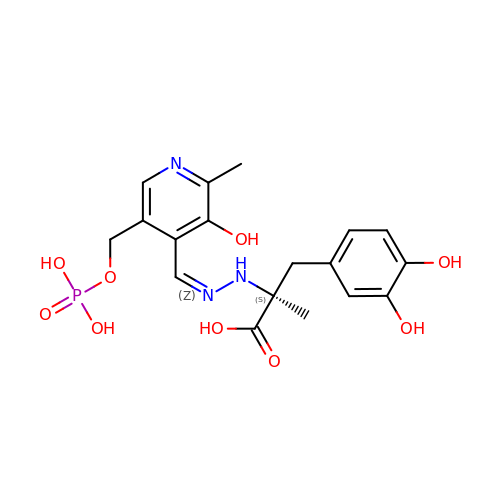(2S)-3-(3,4-dihydroxyphenyl)-2-[(2E)-2-({3-hydroxy-2-methyl-5-[(phosphonooxy)methyl]pyridin-4-yl}methylidene)hydrazin-1-yl]-2-methylpropanoic acid | C18 H22 N3 O9 P | MRJFEJHXBDNBGU-SFHVURJKSA-N> SMACTIQKAEALDGAHLMQILWYDEEESLYPAVWLRDNCPCSDCYLDSAKARKLLVEALDVNIGIKGLIFDRKKVYITWPDEHYSEFQADWLKKRCFSKQARAKLQRELFFPECQYWGSELQLPTLDFEDVLRYDEHAYKWLSTLKKVGIVRLTGASDK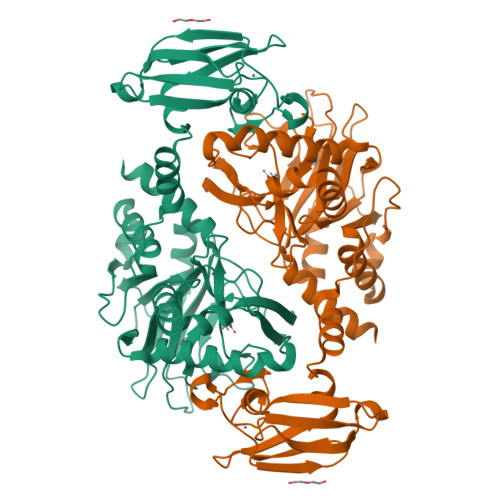PGEVSKLGKRMGFLYLTFYGHTWQVQDKIDANNVAYTTGKLSFHTDYPALHHPPGVQLLHCIKQTVTGGDSEIVDGFNVCQKLKKNNPQAFQILSSTFVDFTDIGVDYCDFSVQSKHKIIELDDKGQVVRINFNNATRDTIFDVPVERVQPFYAALKEFVDLMNSKESKFTFKMNPGDVITFDNWRLLHGRRSYEAGTEISRHLEGAYADWDVVMSRLRILRQRVENGN>[2x]MENTENSVDSKSIKNLEPKIIHGSESMDSGISLDNSYKMDYPEMGLCIIINNKNFHKSTGMTSRSGTDVDAANLRETFRNLKYEVRNKNDLTREEIVELMRDVSKEDHSKRSSFVCVLLSHGEEGIIFGTNGPVDLKKITNFFRGDRCRSLTGKPKLFIIQACRGTELDCGIETDSGVDDDMACHKIPVDA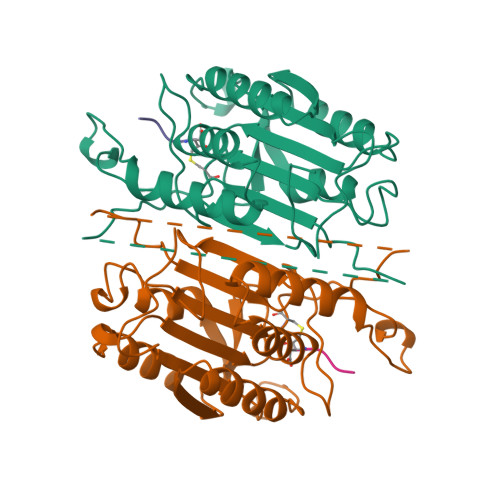DFLYAYSTAPGYYSWRNSKDGSWFIQSLCAMLKQYADKLEFMHILTRVNRKVATEFESFSFDATFHAKKQIPCIVSMLTKELYFYH> SEFMEPLKVEKFATANRGNGLRAVTPLRPGELLFRSDPLAYTVCKGSRGVVCDRCLLGKEKLMRCSQCRVAKYCSAKCQKKAWPDHKRECKCLKSCKPRYPPDSVRLLGRVVFKLMDGAPSESEKLYSFYDLESNINKLTEDRKEGLRQLVMTFQHFMREEIQDASQLPPAFDLFEAFAKVICNSFTICNAEMQEVGVGLYPSISLLNHSCDPNCSIVFNGPHLLLRAVRDIEVGEELTICYLDMLMTSEERRKQLRDQYCFECDCFRCQTQDKDADMLTGDEQVWKEVQESLKKIEELKAHWKWEQVLAMCQAIISSNSERLPDINIYQLKVLDCAMDACINLGLLEEALFYGTRTMEPYRIFFPGSHPVRGVQVMKVGKLQLHQGMFPQAMKNLRLAFDIMRVTHGREHSLIEDL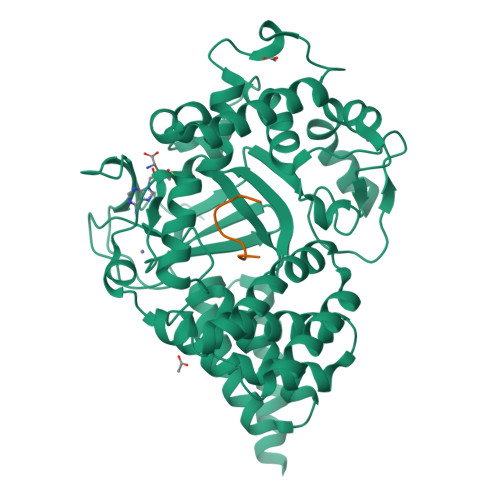ILLLEECDANIRAS;> EKFGKGGTYP> MVKIVYPNAKDFFSFINSITNVTDSIILNFTEDGIFSRHLTEDKVLMAIMRIPKDVLSEYSIDSPTSVKLDVSSVKKILSKASSKKATIELTETDSGLKIIIRDEKSGAKSTIYIKAEKGQVEQLTEPKVNLAVNFTTDESVLNVIAADVTLVGEEMRISTEEDKIKIEAGEEGKRYVAFLMKDKPLKELSIDTSASSSYSAEMFKDAVKGLRGF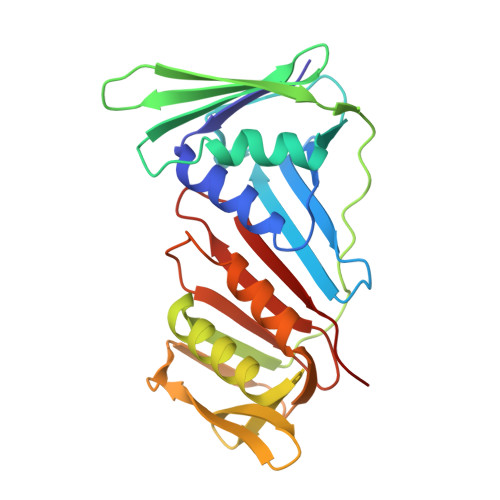SAPTMVSFGENLPMKIDVEAVSGGHMIFWIAPRL3-[(1~{S})-1-[4-azanyl-3-(3-fluoranyl-5-oxidanyl-phenyl)pyrazolo[3,4-d]pyrimidin-1-yl]ethyl]-4-phenyl-isochromen-1-one | C28 H20 F N5 O3 | 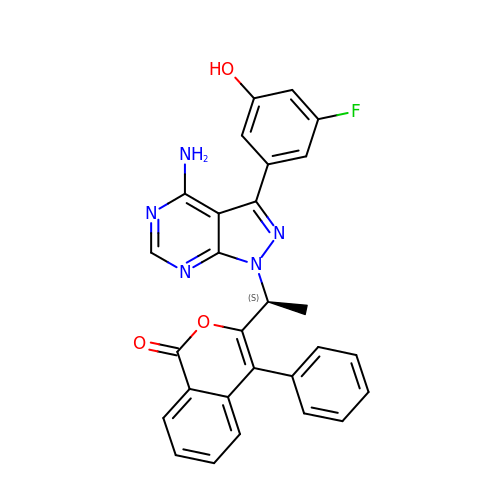JHPVAFKJRDQHCS-HNNXBMFYSA-N> DVYVPDEWEVAREKITMSRELGQGSFGMVYEGVAKGVVKDEPETRVAIKTVNEAASMRERIEFLNEASVMKEFNCHHVVRLLGVVSQGQPTLVIMELMTRGDLKSYLRSLRPEMENNPVLAPPSLSKMIQMAGEIADGMAYLNANKFVHRDLAARNCMVAEDFTVKIGDFGMTRDIYETDYYRKGGKGLLPVRWMSPESLKDGVFTTYSDVWSFGVVLWEIATLAEQPYQGLSNEQVLRFVMEGGLLDKPDNCPDMLFELMRM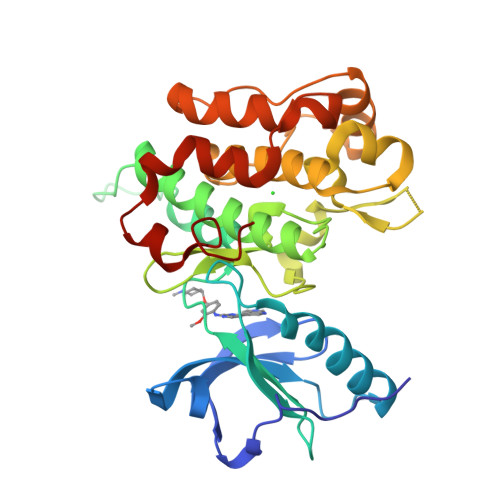CWQYNPKMRPSFLEIISSIKEEMEPGFREVSFYYSEENK>[8x]MDDLTIEILTDDADYDLQRFDCGEEALNLFLTTHLVRQHRNKILRAYILCRNTPERQVLGYYTL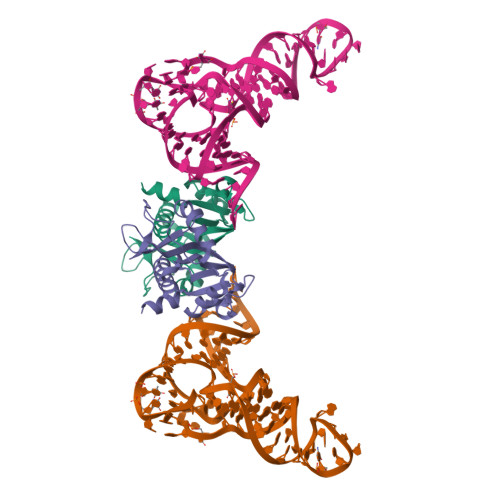CGSCFERAALPSKSKQKKIPYKNIPSVTLGRLAIDRSLQGQGWDATLVAHAMNVVWSASLAVGIHGLFVEALNEKAHTFYKSLGFIPLVGENENALFFPTKSIELLFTQSDLEHHHHHH>[2x]MGSSHHHHHHSQDPMSQQAIGSLETKGFPPILAAADAMVKAGRITIVSYMRAGSARFAVNIRGDVSEVKTAMDAGIEAAKNTPGGTLETWVIIPRPHENVEAVFPIGFGPEVEQYRL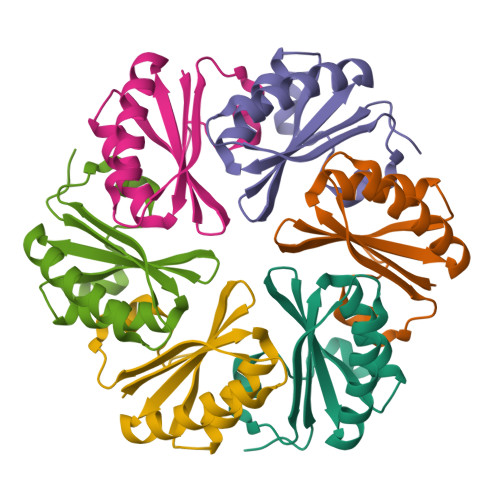SAEGTGSGRR>MMTTGKSDRPRNSVRVGYRGTKFLFVDITKHLLHDGEKEVYVSALGGAINEAVSVVEMLKDQQMVVVKKI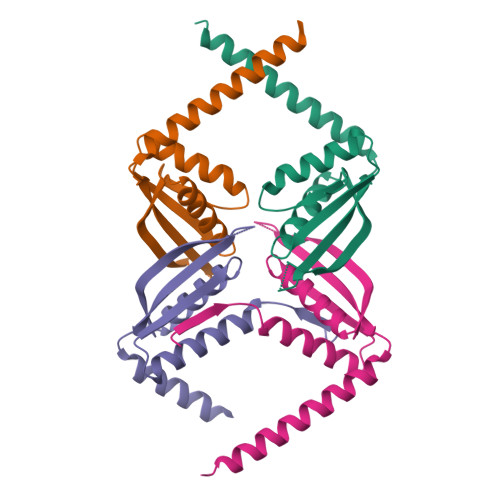TTSRQVSEEPDDGPVDKIEIVVTKADGFDAKYEEQQKAREAKRLEKEKNEKEKATALEHHHHHH[4x]(3E)-N-(2,6-DIETHYLPHENYL)-3-{[4-(4-METHYLPIPERAZIN-1-YL)BENZOYL]IMINO}PYRROLO[3,4-C]PYRAZOLE-5(3H)-CARBOXAMIDE 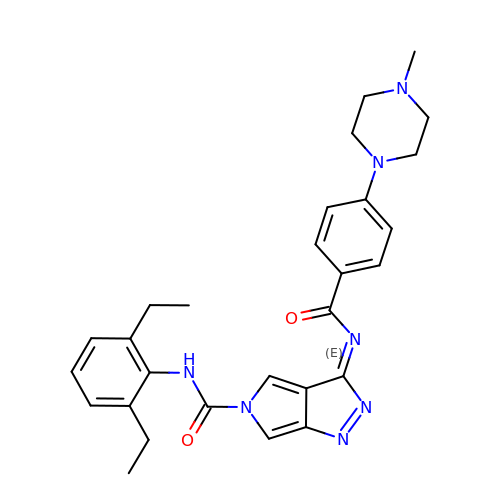| C28 H31 N7 O2 | WUWKQGPEIAHGLN-URGPHPNLSA-N> MPAYSEVKGTCGTPVLDQLIGYYVNIQSRKMYYKDFLRIEHQAVRWAFADIRKNSEALAHGLLQTGVRPGDRVLAIQPCNCETFVLQLSCAKIGALLCIVPQDTISADKLRFYLNEFQPRHLVAREWINVPEMKQGELVERNMHFWDTIYNVIPELGLSYPGQKFQWVHSQEFYYLKKIIITDHNMNLLGVTPMRKMLVWGPFSYYEQRLRRLSALLHPDDPVLALEDPNPAMEDKLHITYSHRNCVNAGFLFGQLMQLKAETRFGVMPNHHTDPIGAIIAPYAALTSGAVLVHIHSDMFTDDHAINGIEKLCVEEVETLVGRKADFDLILKHAGNFDADQFEHLRSVVIFEDGIEAPVSEEYLNKLSKALSLDDVYVFRGPIEASYMLT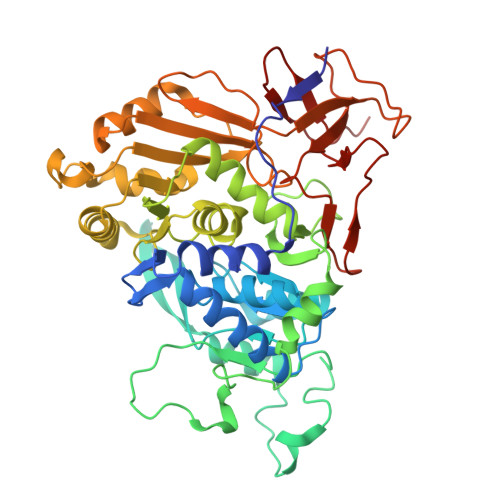WRTLKKGSQGMVPHVEAKVVGDRGTSDAKVLVAGTRGNLRLKGPHVTAGYYNNAGLMTELIDEHGFASTSREAMIDGKDNITLMSAQTY> MNEIVVKGARVHNLKNITVRIPKNRLVVITGVSGSGKSSLAMDTIYAEGQRRYLESLSTYARQFLGNLKKPDVDEIEGLSPAIAIDQKTVSHNPRSTVGTVTEIYDYLRVLYARIGKAHCPECGRPLEKKSIDEILQDLFNSFKEGSRIYILAPVATEKKGTFKKEIEEFISKGFARIEIDGEIYRLEEVPELDKNKRHTVKLVVDRLILETRNEHRILDSLELAMREGKGFVEIRNVDTGESKIFSENLMCPVCGIGFPEITPKLFSFNSPYGACPNCHGLGFTFEVDPSLVIDEEKSVLEGAIIPYRWDRRLSRWVAREIEKRGVSPHLPFKDLPEDVKEFILYGDDRFEGVVPKVQRWHRETESPEMKEWLEKNFIVQRTCSVCGGRRLNREALSVKINGLNIHEFTELSISEELEFLKNLNLTEREREIVGELLKEIEKRLEFLVDVGLEYLTLSRSATTLSGGESQRIRLATQIGSGLTGVIYVLDEPTIGLHPRDT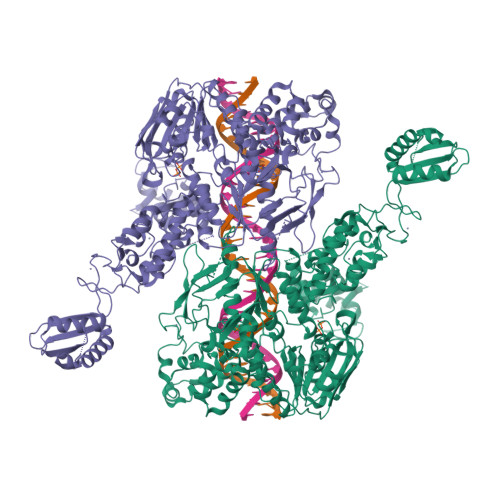ERLIKTLKKLRDLGNTVIVVEHDEEVIRNADHIIDIGPGGGTNGGRVVFQGTVDELLKNPDSSLTGEYLSGKRKITVNKTRRLPYASLKIKGVRHNNLKNIDVEIPLGVFVCVTGVSGSGKSSLVMETLYPALMNLLHKTKLPAGEFDSIEGHENIDKMIAIDQSPIGRTPRSNPATYTKVFDEIRSLFAMTPAAKARGYNKSRFSFNLKGGRCEACQGQGYVKIEMLFLPDVYVECDVCKGKRYNRETLEITYKGKNISDILDMTVDEALEFFKNIPSIKRTLQVLHDVGLGYVKLGQPATTLSGGEAQRIKLASELRKRDTGRTLYILDEPTVGLHFEDVRKLVEVLHRLVDRGNTVIVIEHNLDVIKNADHIIDLGPEGGKEGGYIVATGTPEEIAKNPHSYTGRFLKNVL>STAGKVIKCKAAVLWEEKKPFSIEEVEVAPPKAHEVRIKMVATGICRSDDHVVSGTLVTPLPVIAGHEAAGIVESIGEGVTTVRPGDKVIPLFTPQCGKCRVCKHPEGNFCLKNDLSMPRGTMQDGTSRFTCRGKPIHHFLGTSTFSQYTVVDEISVAKIDAASPLEKVCLIGCGFSTGYGSAVKVAKVTQGSTCAVFGLGGVGLSVIMGCKAAGAARIIGVDINKDKFAKAKEVGATECVNPQDYKKPIQEVLTEMSNGGVDFSFEVIGRLDTMVTALSCCQEAYGVSVIVGVPPDSQNLSMNPMLLLSGRTWKGCIFGGFKSKDSVPKLVADFMAKKFALDPLITHVLPFEKINEGFDLLRSGESIRTILT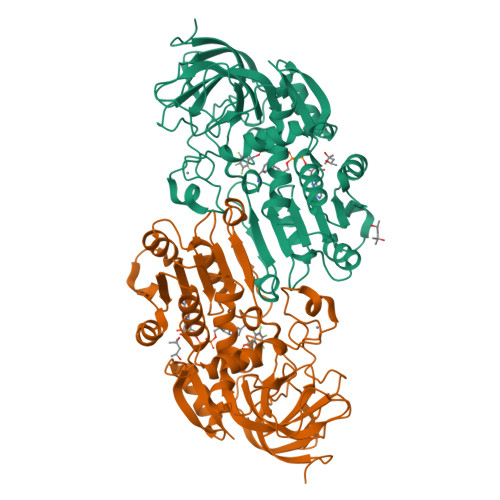F[2x]(2R)-N-[3-(heptylamino)-3-oxopropyl]-2,4-dihydroxy-3,3-dimethylbutanamide | C16 H32 N2 O4 | 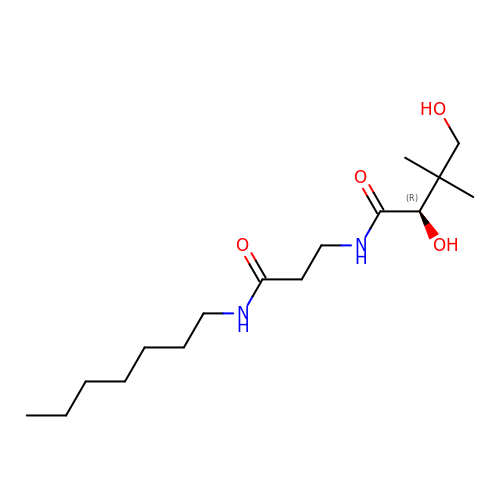HHAVGBXLGVYXFF-AWEZNQCLSA-N> AAAAAAAAAAAAAA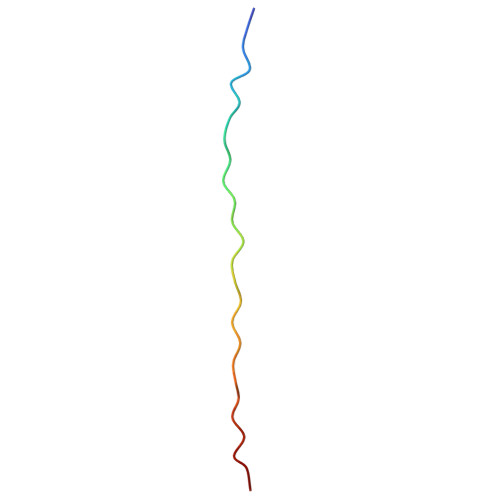AAAAAAAAAAAA>MQDCGLPPDVPNAQPALEGRTSFPEDTVITY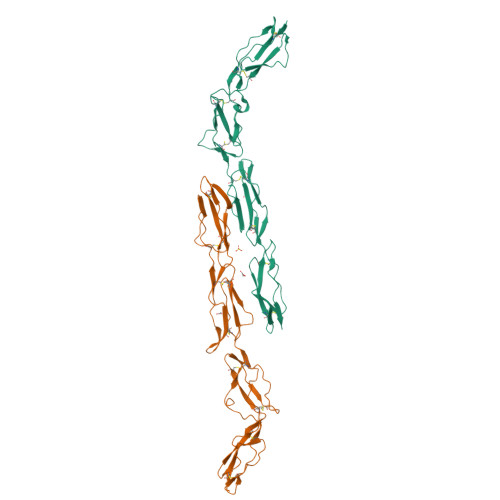KCEESFVKIPGEKDSVICLKGSQWSDIEEFCNRSCEVPTRLNSASLKQPYITQNYFPVGTVVEYECRPGYRREPSLSPKLTCLQNLKWSTAVEFCKKKSCPNPGEIRNGQIDVPGGILFGATISFSCNTGYKLFGSTSSFCLISGSSVQWSDPLPECREIYCPAPPQIDNGIIQGERDHYGYRQSVTYACNKGFTMIGEHSIYCTVNNDEGEWSGPPPECRGC[4x]>KNNDKLTLWTTPDTSPNCRIDQDKDSKLTLVLTKCGSQILANVSLIVVAGRYKIINNNTNPALKGFTIKLLFDKNGVLMESSNLGKSYWNFRNQNSIMSTAYE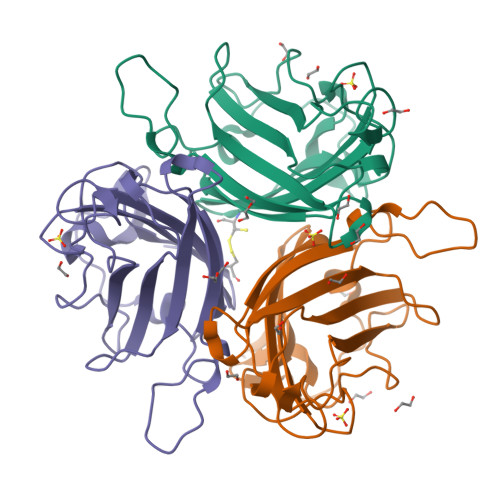KAIGFMPNLVAYPKPTTGSKKYARDIVYGNIYLGGKPHQPVTIKTTFNQETGCEYSITFDFSWAKTYVNVEFETTSFTFSYIAQE[6x]>IIDGAPCARGSHPWQVALLSGNQLHCGGVLVNERWVLTAAHCKMNEYTVHLGSDTLGDRRAQRIKASKSFRHPGYSTQTHVNDLMLVKLNSQARLSSMVKKVRLPSRCEPPGTTCTVSGWGTTTSPDVTFPSDLMCVDVKLISPQDCTKVYKDLLENSMLCAGIP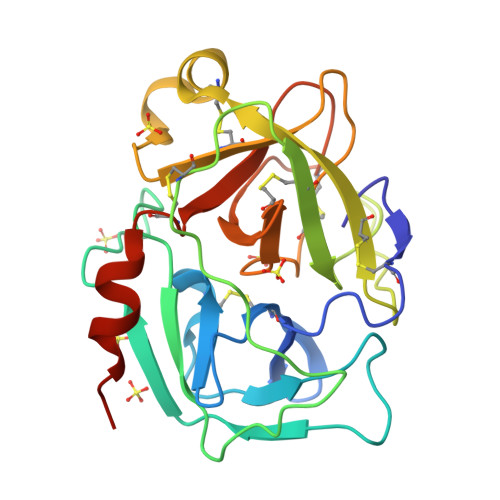DSKKNACNGDSGGPLVCRGTLQGLVSWGTFPCGQPNDPGVYTQVCKFTKWINDTMKHHHHHH[3x]>GSMVNSNNKLTASSLREA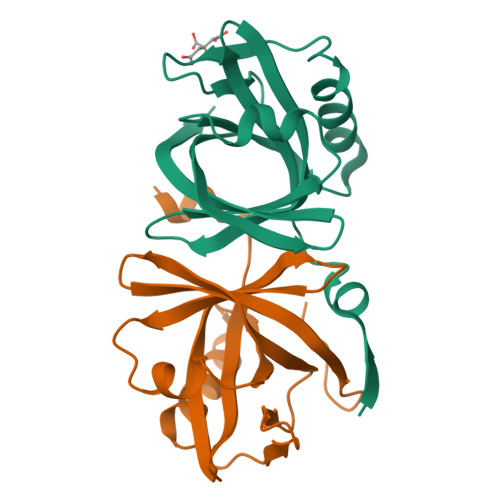FGHFPSGVVAIAAEVNGTLEGLAASTFVPVSLDPPLVSFCVQNTSTTWPKLKDRPMLGISVLGEEHDEAARTLAAKTGDRFAGLETVSRPTGAVFIKGTALWLESAVEQLIPAGDHTIVVLRVNEVTVDANVAPIVFHRSGFRRLGA[2x]>[2x]GTIYPRNPAMYSEEARLKSFQNWPDYAHLTPRELASAGLYYTGIGDQVQCFACGGKLKNWEPGDRAWSEHRRHFPNCFFVLGRNLN;> ATAA

XIAP (X-linked inhibitor of apoptosis) directly inhibits the upstream caspase-9 and the downstream caspase-3 and caspase-7, and therefore controls critical apoptotic checkpoints. The XIAP protein consists of several domains, including three zinc-containing BIR (baculovirus IAP repeat) domains (BIR1, BIR2 and BIR3) and a C-terminal RING domain. The linker region blocks the active sites of these caspases, while the N-terminal regions of the partially processed caspase-3 and caspase-7 bind the BIR2 domain in a peptide-binding groove that accommodates the four N-­terminal residues. As has been reported previously for other BIR domains, the overall architecture of the BIR2 domain is a three-stranded antiparallel β-sheet surrounded by five α-helices, with a structurally important zinc residue coordinated by Cys200, Cys203, His220 and Cys227.

The most potent tetrapeptide among those assayed against BIR2 is ATAA, which interestingly was inactive against BIR3 in our assay. In fact, all peptides with alanine at the P3 position were essentially inactive against BIR3. Therefore, the structures of XIAP BIR2 with five different peptides soaked in and bound to the Smac binding groove were also solved: ATAA, AVPI, SVPI, AIAV and AMRV. As in all described BIR-domain structures, the P1 alanine points to the face of Trp210, which creates the bottom face of the pocket. The N-terminal amino group is anchored by several hydrogen bonds to the surrounding acidic residues Asp214 and Glu219. Arg222, which is poorly resolved in the apo structure, is well resolved in the peptide-bound structure, bending in towards the binding groove to interact with Glu219 and His223. P2 makes standard backbone-to-backbone hydrogen-bond interactions with BIR2, and the side chain points towards solvent. The only interactions are hydrophobic ones with the side chains of Asn209 and Lys208, perhaps leading to the weak preference of BIR2 for hydrophobic residues at P2 (see the AMRV structure), but explaining the general lack of strong preferences for this residue. The P3 alanine is rotated so as to sit along the hydrophobic surface of the protein, and the P4 alanine points into a small pocket created by the side chains of Lys206, Lys208 and Gln197, although Gln197 can rotate away to make a deeper pocket, as will be shown later. Finally, the P4 backbone NH donates a hydrogen bond to the backbone of Lys206.>[4x]GSMKQPFERILREICFMVKVEGRKVLRDFGITPAQFDILQKIYFEGPKRPGELSVLLGVAKSTVTGLVKRLEADGYLTRTPDPADRRAYFLVITRKGEEVIE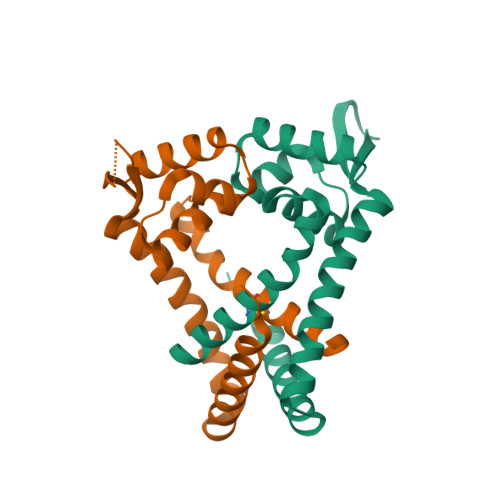KVIERRENFIEKITSDLGKEKSSKILDYLKELKGVMERNFSKQ>GASRPVVSGVASLGYEEQEVLKMAAAVEKTATHPIAKAIVNEAESLNLKTPETRGQLTEPGFGTLAEIDGRFVAVGSLEWVSDRFLKKNDSSDMVKLESLLDHKLSNTSSTSRYSKTVVYVGREGEGIIGAIAISD[2x]

P-type ATPases are transmembrane proteins that play a key role in the uphill transport of a wide range of cations across membranes using the energy provided by the hydrolysis of ATP, being crucial for the ion homeostasis in nearly all organisms and for heavy metal detoxification. HMA1 and HMA6 are found in the inner membrane of the chloroplast envelope and HMA8 in the thylakoid membrane. Here, we present two structures of the nucleotide binding domain of HMA6 and HMA8, the former at the highest resolution, obtained for any P-type ATPase structure. The overall structure of HMA6N-AA and HMA8N (respectively) exhibits a twisted, antiparallel β-sheet made of six strands being flanked by two pairs of short α-helices, one on the concave (α1 and α2) and one on the convex (α3 and α4) side of the sheet.

HMA8 supplies plastocyanin in the thylakoid lumen with copper, which also controls the stability of HMA8, but not of HMA6. However, they exhibit differing catalytic properties, HMA8 having a higher affinity for Cu and lower dephosphorylation kinetics than HMA6. The N-domain of HMA8 (HMA8N) was readily expressed and purified, representing monomeric protein, which eluted as a symmetric peak with a calculated mass of 17.2 kDa. For both proteins, two molecules are present in the AU, yet they are monomeric in solution as found by size exclusion chromatography. The position of the second missing loop is identical in both structures, differing only in the length, as in HMA8 an insertion is present, not typically found in the subfamily. Furthermore, the insertion found in HMA8 could interact tighter with the P-domain and report on the N-domain inclination. In parallel, several attempts to obtain the structure of the HMA N-domains in complex with ATP were made by soaking or co-crystallization on HMA8N. They led to diffracting crystals but no density of the nucleotide could be observed. Of interest is also a second salt bridge in the vicinity of the nucleotide binding domain, E673-R697 in HMA6 and E612-R637 in HMA8, linking β2 to α3. Marked differences between ATP/ADP ratios in the cytosol and the chloroplast stroma, as well as between the pH of these two subcellular compartments (increase of the stromal alkalization on illumination), might also explain differences in electrostatic properties of this surface (HMA8 requires the efficient use of ATP at a low ATP/ADP ratio found in the stroma).> AEAGITGTWYAQLGD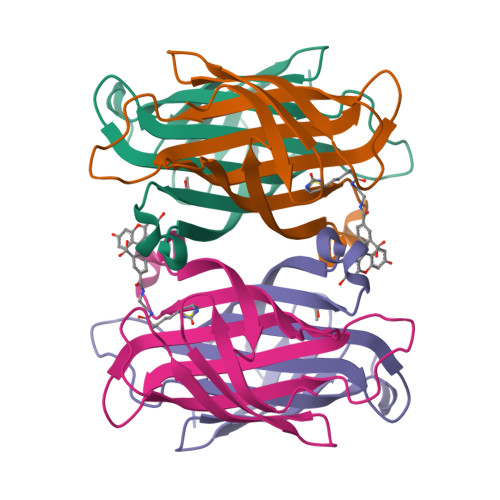TFIVTAGADGALTGTYEAAVGNAESRYVLTGRYDSAPATDGSGTALGWTVAWKNNYRNAHSATTWSGQYVGGAEARINTQWLLTSGTTEANAWKSTLVGHDTFTKVKPSAASA;> AEAGITGTWYNQLGSTFIVTAGADGALTGTYESAVGNAESRYVLTGRYDSAPATDGSGTALGWTVAWKNNYRNAHSATTWSGQYVGGAEARINTQWLLTSGTTEANAWKSTLVGHDTFTKVKPSAASEEEEEE>[4x]MAQERKVALVTGASRGIGAAIAQQLIQDGYFVVGTATSESGAQKLTDSFGEQGAGLALDVRNLDEIEAVVSHIEQNYGPVLVLVNNAGITKDN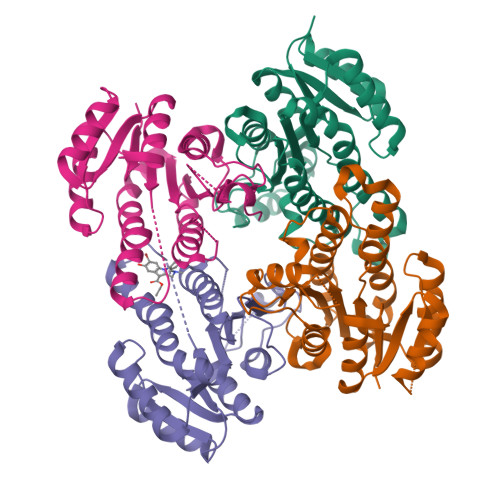LLLRMSEDDWDDILNIHLKAVYRLSKRVLKGMTKARFGRIINISSVVAHFANPGQANYSAAKAGIEAFSRSLAKEMGSRQITVNSVAPGFIATEMTDALSEDIRKKMSDQVALNRLGEPQDIANAVSFLASDKAGYITGTVLHVNGGLYMA> GSHH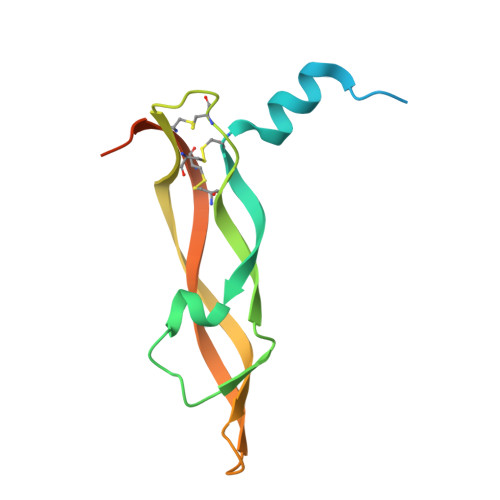HHHHGSAPMAEGGGQNHHEVVKFMDVYQRSYCHPIETLVDIFQEYPDEIEYIFKPSCVPLMRCGGCCNDEGLECVPTEESNITMQIMRIKPHQGQHIGEMSFLQHNKCECRPKKDRARQENCDKPRR The prototypical hydrogen-producing enzyme, the membrane-bound formate hydrogenlyase (FHL) complex from Escherichia coli, links formate oxidation at a molybdopterin-containing formate dehydrogenase to proton reduction at a [NiFe] hydrogenase. As the pH of the growth medium drops, formate re-enters the cell and synthesis of the formate-hydrogen lyase (FHL) complex is induced. This heptameric membrane-bound complex catalyzes the disproportionation of formate to CO2 and H2 allowing efficient production of hydrogen from biomass, a process that was first described over 100 years ago5. The FHL complex exhibits the characteristic L-shaped structure of the complex I superfamily with membrane-embedded and soluble arms. An electron relay containing eight [4Fe4S] clusters, coordinated by FdhF (A1), HycB (B1-B4), HycF (F1, F2) and HycG (G1), leads from the molybdopterin site to a [NiFe] hydrogenase active site in HycE.

The structure of aerobically isolated FHL, determined to 3.4 Å resolution (focused refinements 3.0–3.4 Å) by cryo-EM single-particle analysis provided important detail on the organization of the heptameric complex. However, the map density for the hydrogenase [NiFe] active site and proximal iron-sulfur cluster G1 was weak and poorly resolved, which we attribute to oxidative damage. The size exclusion chromatography (SEC) elution profile of the aerobically isolated complex shows two major peaks, the slower-eluting of which corresponds to a soluble complex lacking the membrane-associated subunits HycC and HycD. Our cryo-EM map obtained from aerobically prepared sample shows a Mo(MGD)2 geometry similar to the crystal structure of oxidized FdhF in the [Mo(VI)]-state. FdhF interacts with HycB via hydrophobic interactions and hydrogen bonds (H-bonds) and with HycF electrostatically. The C-terminal extension of HycF interacts with HycB and contains a cysteine quartet (Cys117, Cys120, Cys155 and Cys158) that coordinates an unpredicted cofactor at the periphery of the protein, consistent with a single metal ion that we have tentatively assigned as iron. Arg122 of HycF, which is near to the ion, exhibits two alternate conformations in the aerobically isolated structure: one facing toward the ion and the other toward the acidic patch of FdhF. In the map obtained from aerobically prepared sample only weak density was observed for the ND1 and β1-β2 loops. We suggest that oxidative damage to the [NiFe] site causes disorder in this region, leading to the partial dissociation of the membrane arm observed by SEC. Our data suggest that FdhF is more strongly associated with the Hyc subunits under oxidizing than under reducing conditions.

> MKKVVTVCPYCASGCKINLVVDNGKIVRAEAAQGKTNQGTLCLKGYYGWDFINDTQILTPRLKTPMIRRQRGGKLEPVSWDEALNYVAERLSAIKEKYGPDAIQTTGSSRGTGNETNYVMQKFARAVIGTNNVDCCARVUHGPSVAGLHQSVGNGAMSNAINEIDNTDLVFVFGYNPADSHPIVANHVINAKRNGAKIIVCDPRKIETARIADMHIALKNGSNIALLNAMGHVIIEENLYDKAFVASRTEGFEEYRKIVEGYTPESVEDITGVSASEIRQAARMYAQAKSAAILWGMGVTQFYQGVETVRSLTSLAMLTGNLGKPHAGVNPVRGQNNVQGACDMGALPDTYPGYQYVKDPANREKFAKAWGVESLPAHTGYRISELPHRAAHGEVRAAYIMGEDPLQTDAELSAVRKAFEDLELVIVQDIFMTKTASAADVILPSTSWGEHEGVFTAADRGFQRFFKAVEPKWDLKTDWQIISEIATRMGYPMHYNNTQEIWDELRHLCPDFYGATYEKMGELGFIQWPCRDTSDADQGTSYLFKEKFDTPNGLAQFFTCDWVAPIDKLTDEYPMVLSTVREVGHYSCRSMTGNCAALAALADEPGYAQINTEDAKRLGIEDEALVWVHSRKGKIITRAQVSDRPNKGAIYMTYQWWIGACNELVTENLSPITKTPEYKYCAVRVEPIADQRAAEQYVIDEYNKLKTRLREAALA;> MNRFVIADSTLCIGCHTCEAACSETHRQHGLQSMPRLRVMLNEKESAPQLCHHCEDAPCAVVCPVNAITRVDGAVQLNESLCVSCKLCGIACPFGAIEFSGSRPLDIPANANTPKAPPAPPAPARVSTLLDWVPGIRAIAVKCDLCSFDEQGPACVRMCPTKALHLVDNTDIARVSKRKRELTFNTDFGDLTLFQQAQSGEAK;> MSAISLINSGVAWFVAAAVLAFLFSFQKALSGWIAGIGGAVGSLYTAAAGFTVLTGAVGVSGALSLVSYDVQISPLNAIWLITLGLCGLFVSLYNIDWHRHAQVKCNGLQINMLMAAAVCAVIASNLGMFVVMAEIMALCAVFLTSNSKEGKLWFALGRLGTLLLAIACWLLWQRYGTLDLRLLDMRMQQLPLGSDIWLLGVIGFGLLAGIIPLHGWVPQAHANASAPAAALFSTVVMKIGLLGILTLSLLGGNAPLWWGIALLVLGMITAFVGGLYALVEHNIQRLLAYHTLENIGIILLGLGAGVTGIALEQPALIALGLVGGLYHLLNHSLFKSVLFLGAGSVWFRTGHRDIEKLGGIGKKMPVISIAMLVGLMAMAALPPLNGFAGEWVIYQSFFKLSNSGAFVARLLGPLLAVGLAITGALAVMCMAKVYGVTFLGAPRTKEAENATCAPLLMSVSVVALAICCVIGGVAAPWLLPMLSAAVPLPLEPANTTVSQPMITLLLIACPLLPFIIMAICKGDRLPSRSRGAAWVCGYDHEKSMVITAHGFAMPVKQAFAPVLKLRKWLNPVSLVPGWQCEGSALLFRRMALVELAVLVVIIVSRGA;> MSVLYPLIQALVLFAVAPLLSGITRVARARLHNRRGPGVLQEYRDIIKLLGRQSVGPDASGWVFRLTPYVMVGVMLTIATALPVVTVGSPLPQLGDLITLLYLFAIARFFFAISGLDTGSPFTAIGASREAMLGVLVEPMLLLGLWVAAQVAGSTNISNITDTVYHWPLSQSIPLVLALCACAFATFIEMGKLPFDLAEAEQELQEGPLSEYSGSGFGVMKWGISLKQLVVLQMFVGVFIPWGQMETFTAGGLLLALVIAIVKLVVGVLVIALFENSMARLRLDITPRITWAGFGFAFLAFVSLLAA;> MSEEKLGQHYLAALNEAFPGVVLDHAWQTKDQLTVTVKVNYLPEVVEFLYYKQGGWLSVLFGNDERKLNGHYAVYYVLSMEKGHHHHHHHHHHGSTKCWITVRVEVDANKPEYPSVTPRVPAAVWGEREVRDMYGLIPVGLPDERRLVLPDDWPDELYPLRKDSMDYRQRPAPTTDAETYEFINELGDKKNNVVPIGPLHVTSDEPGHFRLFVDGENIIDADYRLFYVHRGMEKLAETRMGYNEVTFLSDRVCGICGFAHSTAYTTSVENAMGIQVPERAQMIRAILLEVERLHSHLLNLGLACHFTGFDSGFMQFFRVRETSMKMAEILTGARKTYGLNLIGGIRRDLLKDDMIQTRQLAQQMRREVQELVDVLLSTPNMEQRTVGIGRLDPEIARDFSNVGPMVRASGHARDTRADHPFVGYGLLPMEVHSEQGCDVISRLKVRINEVYTALNMIDYGLDNLPGGPLMVEGFTYIPHRFALGFAEAPRGDDIHWSMTGDNQKLYRWRCRAATYANWPTLRYMLRGNTVSDAPLIIGSLDPCYSCTDRMTVVDVRKKKSKVVPYKELERYSIERKNSPLK;> MFTFIKKVIKTGTATSSYPLEPIAVDKNFRGKPEQNPQQCIGCAACVNACPSNALTVETDLATGELAWEFNLGHCIFCGRCEEVCPTAAIKLSQEYELAVWKKEDFLQQSRFALCNCRVCNRPFAVQKEIDYAIALLKHNGDSRAENHRESFETCPECKRQKCLVPSDRIELTRHMKEAI;> MSNLLGPRDANGIPVPMTVDESIASMKASLLKKIKRSAYVYRVDCGGCNGCEIEIFATLSPLFDAERFGIKVVPSPRHADILLFTGAVTRAMRSPALRAWQSAPDPKICISYGACGNSGGIFHDLYCVWGGTDKIVPVDVYIPGCPPTPAATLYGFAMALGLLEQKIHARGPGELDEQPAEILHGDMVQPLRVKVDREARRLAGYRYGRQIADDYLTQLGQGEEQVARWLEAENDPRLNEIVSHLNHVVEEARIR> TPVMQTIVVKNVPTTIGDTVYITGNRAELGSWDTKQYPIQLYYDS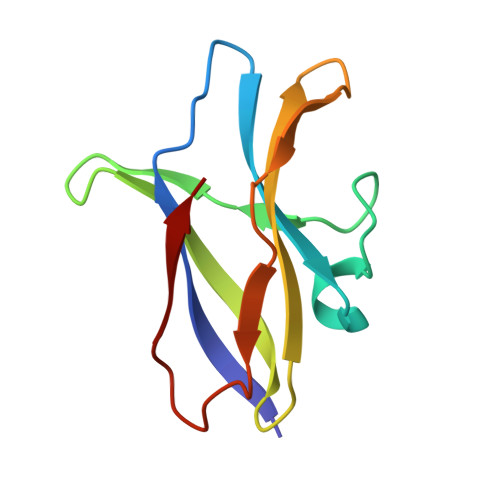HSNDWRGNVVLPAERNIEFKAFIKSKDGTVKSWQTIQQSWNPVPLKTTSHTSSW METHYL (5-{4-[({[2-FLUORO-5-(TRIFLUOROMETHYL)PHENYL]AMINO}CARBONYL)AMINO]PHENOXY}-1H-BENZIMIDAZOL-2-YL)CARBAMATE | C23 H17 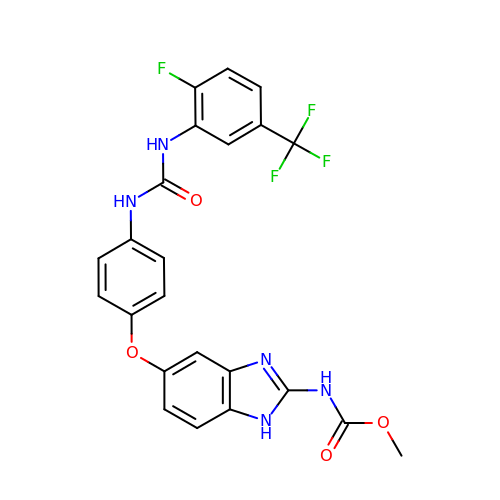F4 N5 O4 | KADQEUOYNAPXRD-UHFFFAOYSA-N> M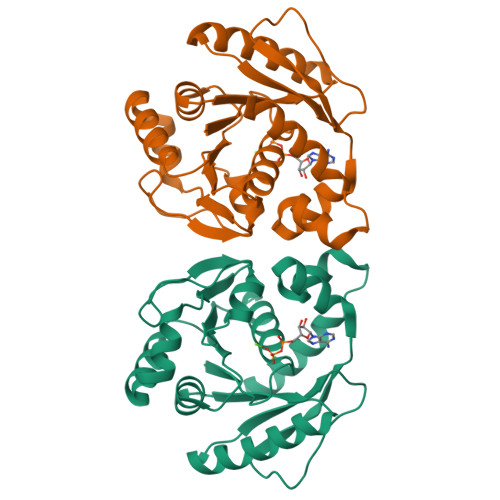IVTVINQKGGVGKTTTSVNLSYYLSKEKKTGLLDLDPEGGATISYGMKRELKELPLGEKSVNIFNVEVFPAHIGLLKLELNGDVEEISNKIKEIGKQFDFLVIDTPPNLGTLAISAMLVADRIVSPVTPQPLALEAIKNLDSRLKSIGKNAYSFTNFSKKVVKLDNLSSVKFTEITIPPSRLFIEASRLGVPALRYEEVRIKKPKLANYYQQLAKVISE> GSHMINVNKKALGQDTEKMEEQLDLLSAILDPSKSKGAGS;> MKGTDFVHSVKKFLRVRIFTKIESEDDYILSGESVMDRDSESEEAETKDIRKQIQLLKKIIFEKELMYQIKKECALLISYGVSIENENKVIIELPNEKFEIELLSLDDDSIVNHEQDLPKINDKRANLMLVMLRLLLVVIFKKTLRSRISSPHGLINLNVDDDILIIRPILGKVRFANYKLLLKKIIKDYVLDIVPGSSITETEVEREQPQENKNIDDENITKLNKEIRAFDKLLNIPRRELKINLPLTEHKSP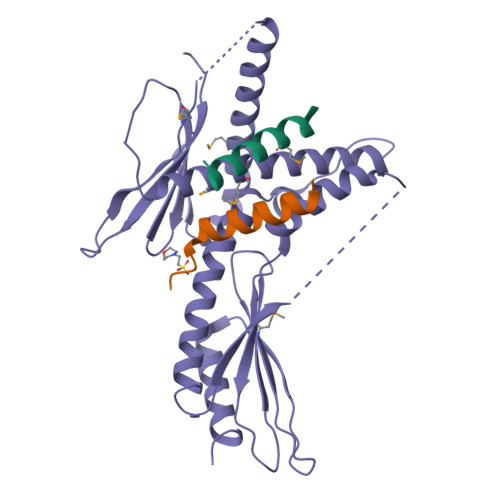NLSLMLESPNYCNALIHIKFSAGTEANAVSFDTTFSDFKEVEDFLHFIVAEYIQQKKV;> GAGSGVTRFDEKQIEELLDNCIETFVAEKTT> GSHMSYNNIPAGKDAPNDIYVIIEIPANAAPIKYEIDKDSDALFVDRFMGTA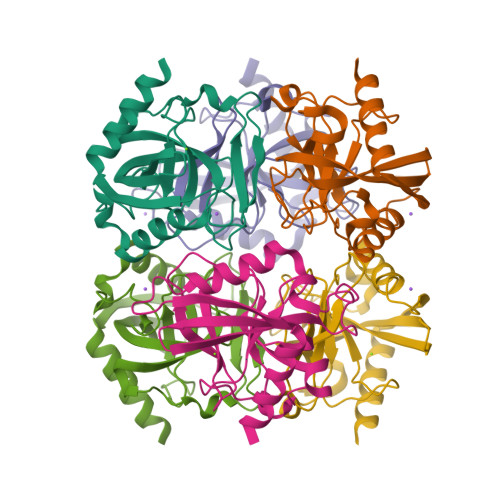MFYPANYGYVPNTLSEDGDPLDVLVVTPYPVAAGSVIRCRPVGKLNMEDDGGIDAKLIAVPHEKLSPLYKDVKEYTDLPQLLINQVEHFFSHYKDLEPGKWVKISGWEGADVAKAEVIKAIEAAK> SPEIMKDLSINFGKALDTCKKELDLPDSINEDFYKFWKEDYEITNRLTGCAIKCLSEKLEMVDADGKLHHGNAREFAMKHGADDAMAKQLVDLIHGCEKSIPPNDD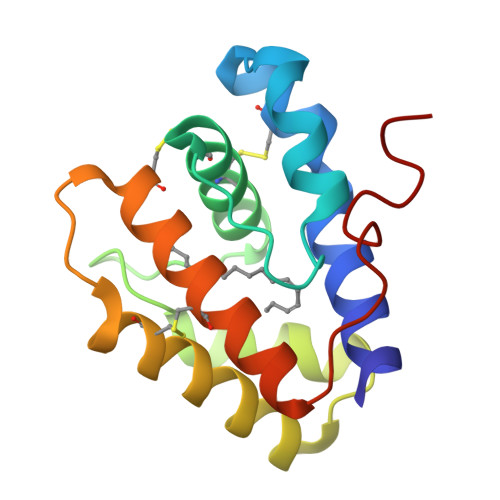RCMEVLSIAMCFKKEIHNLKWAPNMEVVVGEVLA> MLRDLFDRAVVLSHYIHNLSSEMFSEFDKRYTHGRGFITKAINSCHTSSLATPEDKEQAQQMNQKDFLSLIVSILRSWNEPLYHLVTEVRGMQEAPEAILSKAVEIEEQTKRLLERMELIVSQVHPETKENEIYPVWSGLPSLQMADEESRLSAYYNLLHCLRRDSHKIDNYLKLLKCRIIHNNNC;> MLP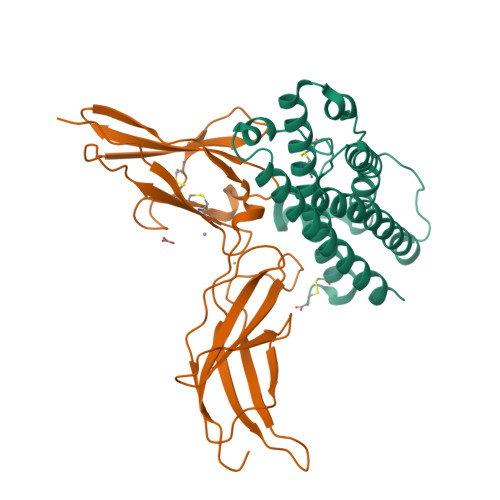PGKPEIFKCRSPNKETFTCWWRPGTDGGLPTNYSLTYHREGETLMHECPDYITGGPNSCHFGKQYTSMWRTYIMMVNATNQMGSSFSDELYVDVTYIVQPDPPLELAVEVKQPEDRKPYLWIKWSPPTLIDLKTGWFTLLYEIRLKPEKAAEWEIHFAGQQTEFKILSLHPGQKYLVQVRCKPDAGYWSAWSPATFIQIPSDFTMND> MSNKNVNVRKSQEITFCLLAGILMFMAMMVAGRAEAGVALGATRVIYPAGQKQEQLAVTNNDENSTYLIQSWVENADGVKDGRFIVTPPLFAMKGKKENTLRILDATNNQLPQD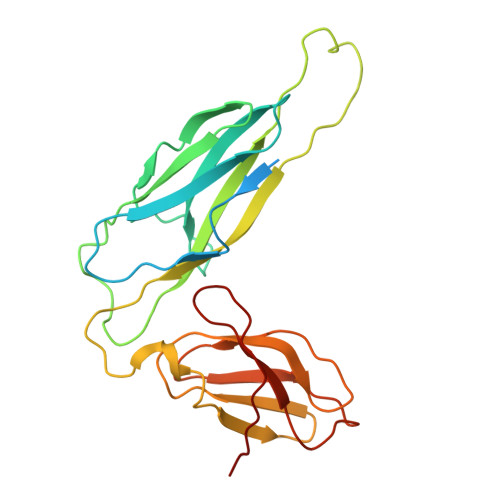RESLFWMNVKAIPSMDKSKLTENTLQLAIISRIKLYYRPAKLALPPDQAAEKLRFRRSANSLTLINPTPYYLTVTELNAGTRVLENALVPPMGESTVKLPSDAGSNITYRTINDYGALTPKMTGVME> APGSVVELLGKSYPQDDHSNLTRKVLTRVGRNLHNQQHHPLWLIKERVKEHFYKQYVGRFGTP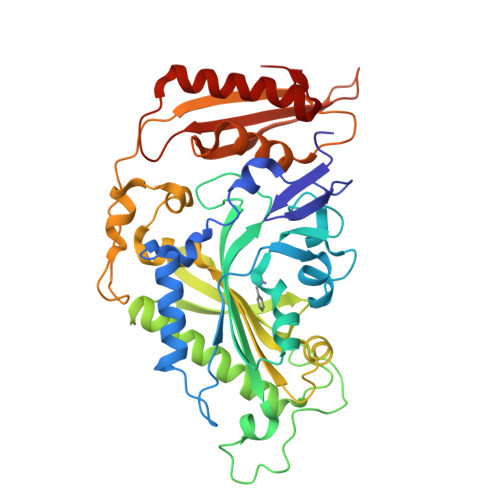LFSVYDNLSPVVTTWQNFDSLLIPADHPSRKKGDNYYLNRTHMLRAHTSAHQWDLLHAGLDAFLVVGDVYRRDQIDSQHYPIFHQLEAVRLFSKHELFAGIKDGESLQLFEQSSRSAHKQETHTMEAVKLVEFDLKQTLTRLMAHLFGDELEIRWVDCYFPFTHPSFEMEINFHGEWLEVLGCGVMEQQLVNSAGAQDRIGWAFGLGLERLAMILYDIPDIRLFWCEDERFLKQFCVSNINQKVKFQPLSKYPAVINDISFWLPSENYAENDFYDLVRTIGGDLVEKVDLIDKFVHPKTHKTSHCYRITYCHMERTLSQREVRHIHQALQEAAVQLLGVEGRF N-[3-[(4S,6S)-2-azanyl-4-methyl-6-(trifluoromethyl)-5,6-dihydro-1,3-thiazin-4-yl]-4-fluoranyl-phenyl]-5-(fluoranylmethoxy)pyrazine-2-carboxamide 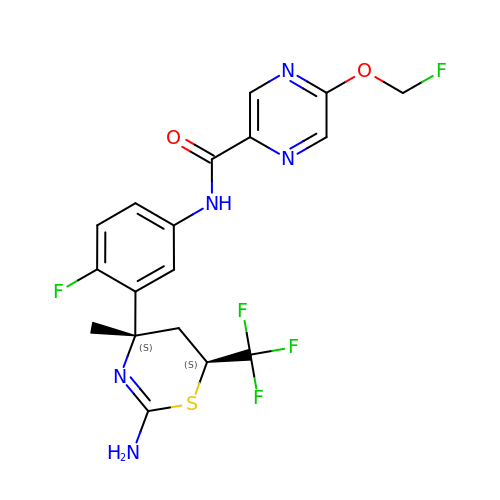| C18 H16 F5 N5 O2 S | JRPAQOLQALFUAQ-GUYCJALGSA-N>[4x]MLPVEGSEEDKSQTGVNRASKGG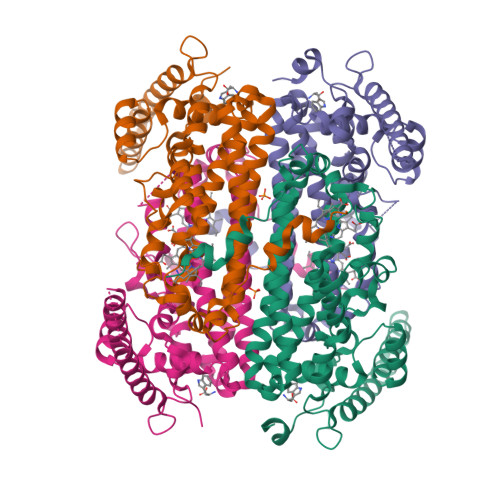LIYGNYLHLEKVLNAQELQSETKGNKIHDEHLFIITHQAYELWFKQILWELDSVREIFQNGHVRDERNMLKVVSRMHRVSVILKLLVQQFSILETMTALDFNDFREYLSPASGFQSLQFRLLENKIGVLQNMRVPYNRRHYRDNFKGEENELLLKSEQEKTLLELVEAWLERTPGLEPHGFNFWGKLEKNITRGLEEEFIRIQAKEESEEKEEQVAEFQKQKEVLLSLFDEKRHEHLLSKGERRLSYRALQGALMIYFYREEPRFQVPFQLLTSLMDIDSLMTKWRYNHVCMVHRMLGSKAGTGGSSGYHYLRSTVSDRYKVFVDLFNLSTYLIPRHWIPKMNPTIHKFLEHHHHHH> MPKVTDIANELKQAIDAKDEVQIAFIASEYSAESREKIAKAYVASYGKELPDDIK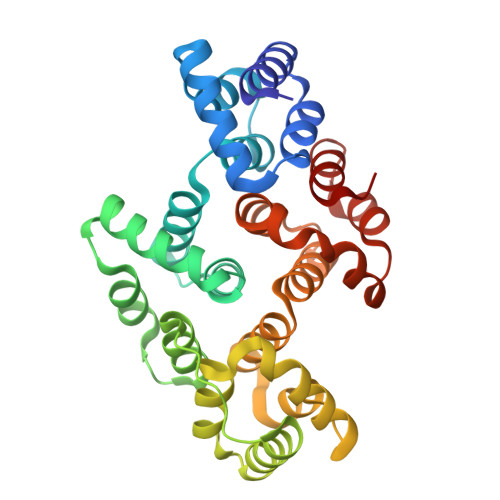KALKGGSEESLLMDLFSDRHEVRAQHIRDALSGRNDHMAFFDTVILCTPEDWHETVAAYTRMFKKPLVEDFMKDVGRKEDWCLLMEKWMAHERVSRPGSPEDEAQRLDQAFDQKNTAYLIDFFGTVPSAEYRPIAEAFKAQNGKSIEQAIATIYTKTDYYTFYCAHFALLGMHRLAAYLINCACNDKGDEKRMRRITGMMVDKCLGAKHAYKIYGDMGTDIERCFDKRMAPILRTLWRVK N-SUCCINYL LYSINE | C10 H18 N2 O5 | 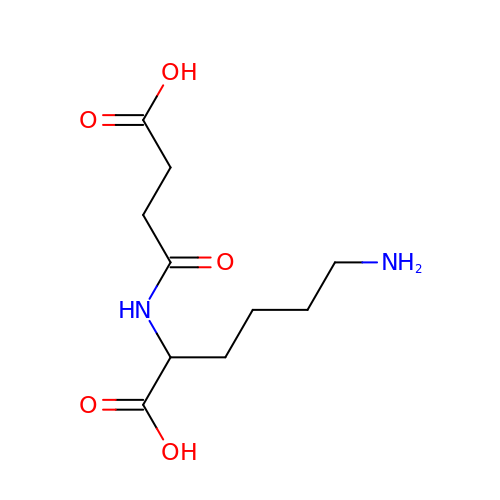XEOGRHZGJFTETQ-ZETCQYMHSA-N> GAMGGSMIKGKLMPNSLKDVQ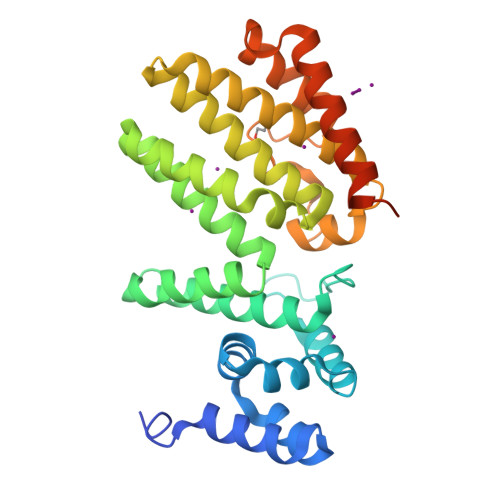KLICDEGITDNVITTLSRLKPFDLAMLKATSDNKVKTLLDSDELKPFWVNKFNKLRLEKDHIFQFRNPDPQSRADFYCGYVLYLAALKEKQKEISSYYDYLNLSFTTFNCFYAAQEILTFLIGACKNDTKRENIDLLYNFVTSQSTQIQEHKTPGCLLLANAYFYLAGFYLSLDLKAESIECYKECWGQLHLAQLLETDSEREIHNAYFNKGLATSNAFGLNSISEIKARCLDLASEALPYPARNVMEANAVKTFENRFKDSMSTAGKDDERSITRPIIL>NIFEXQVDAQPLRPCELQRERAFLKREDYVPQCAEDGSFQTVQCGKDGASCWCVDADGREVPGSRQPGRPAACLSFCQLQKQQILLSSYINSTATSYLPQCQDSGDYSPVQCDLRRRQCWCVDAEGMEVYGTRQQGRPARCPRSCEIRNRRLLHGVGDRSPPQCSPDGAFRPVQCKFVNTTDMMIFDLVHSYSRFPDAFVTFSSFRSRFPEVSGYCYCADSQGRELAETGLELLLDEIYDTIFAGLDLASTFAETTLYRILQRRFLAVQLVISGRFRCPTKCEVERFAATSFRHPYVPSCHPDGEYQAAQCQQGGPCWCVDSRGQEIPGTRQRGEPPSCAEDQSCPSERRRAFSRLRFGPSGYFSRRSLLLAPEEGPVSQRFARFTASCPPSIKELFLDSGIFQPMLQGRDTRFVAPESLLKEAIRGLFPSRELARLALQFTTNAKRLQQNLFGGRFLVNVGQFNLSGALGTRGTFNFSHFFQQLGLPGFQDGRALADLAKPLSVGLNSNPASEAPKASKIDVALRKPVVGSFGFEVNLQENQNALQFLSSFLELPEFLLFLQHAISVPEDIARDLGDVMEMVFSSQGCGQAPGSLFVPACTAEGSYEEVQCFAGDCWCVDAQGRELAGSRVRGGRPRCPTECEKQRARMQSLLGSQPAGSSLFVPACTSKGNFLPVQCFNSECYCVDTEGQPIPGTRSALGEPKKCPSPCQLQAERAFLGTVRTLVSNPSTLPALSSIYIPQCSASGQWSPVQCDGPPEQAFEWYERWEAQNSAGQALTPAELLMKIMSYREAASRNFRLFIQNLYEAGQQGIFPGLARYSSFQDVPVSVLEGNQTQPGGNVFLEPYLFWQILNGQLDRYPGPYSDFSAPLAHFDLRSCWCVDEAGQKLEGTRNEPNKVPACPGSCEEVKLRVLQFIREAEEIVTYSNSSRFPLGESFLAAKGIRLTDEELAFPPLSPSRETFLEKFLSGSDYAIRLAAQSTFDFYQRRLVTLAESPRAPSPVWSSAYLPQCDAFGGWEPVQCHAATGHCWCVDGKGEYVPTSLTARSRQIPQCPTSCERLRASGLLSSWKQAGVQAEPSPKDLFIPTCLETGEFARLQASEAGTWCVDPASGEGVPPGTNSSAQCPSLCEVLQSGVPSRRTSPGYSPACRAEDGGFSPVQCDPAQGSCWCVLGSGEEVPGTRVAGSQPACESPQCPLPFSVADVAGGAILCERASGLGAAAGQRCQLRCSQGYRSAFPPEPLLCSVQRRRWESRPPQPRACQRPQFWQTLQTQAQFQLLLPLGKVCSADYSGLLLAFQVFLLDELTARGFCQIQVKTAGTPVSIPVCDDSSVKVECLSRERLGVNITWKLQLVDAPPASLPDLQDVEEALAGKYLAGRFADLIQSGTFQLHLDSKTFSADTSIRFLQGDRFGISPRTQFGCLEGFGRVVAASDASQDALGCVKCPEGSYFQDEQCIPCPAGFYQEQAGSLACVPCPEGRTTVYAGAFSQTHCVTDCQKNEVGLQCDQDGQYRASQRDRTSGKAFCVDGEGRRLPWTEAEAPLVDAQ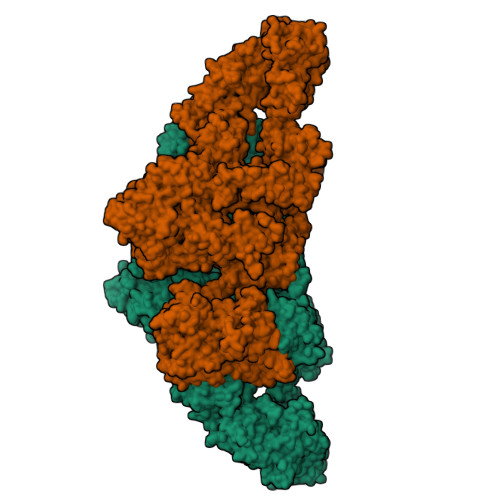CLVMRKFEKLPESKVIFSADVAVMVRSEVPGSESSLMQCLADCALDEACGFLTVSTAGSEVSCDFYAWASDSIACTTSGRSEDALGTSQATSFGSLQCQVKVRSREGDPLAVYLKKGQEFTITGQKRFEQTGFQSALSGMYSPVTFSASGASLAEVHLFCLLACDHDSCCDGFILVQVQGGPLLCGLLSSPDVLLCHVRDWRDPAEAQANASCPGVTYDQDSRQVTLRLGGQEIRGLTPLEGTQDTLTSFQQVYLWKDSDMGSRSESMGCRRDTEPRPASPSETDLTTGLFSPVDLIQVIVDGNVSLPSQQHWLFKHLFSLQQANLWCLSRCAGEPSFCQLAEVTDSEPLYFTCTLYPEAQVCDDILESSPKGCRLILPRRPSALYRKKVVLQDRVKNFYNRLPFQKLTGISIRNKVPMSDKSISSGFFECERLCDMDPCCTGFGFLNVSQLKGGEVTCLTLNSLGLQTCSEEYGGVWRILDCGSPDTEVRTYPFGWYQKPVSPSDAPSFCPSVALPALTENVALDSWQSLALSSVIVDPSIRNFDVAHISTAAVGNFSAARDRCLWECSRHQDCLVTTLQTQPGAVRCMFYADTQSCTHSLQAQNCRLLLHEEATYIYRKPNIPLPGFGTSSPSVPIATHGQLLGRSQAIQVGTSWKPVDQFLGVPYAAPPLGEKRFRAPEHLNWTGSWEATKPRARCWQPGIRTPTPPGVSEDCLYLNVFVPQNMPPNASVLVFFHNAAEGKGSGDRPAVDGSFLAAVGNLIVVTASYRTGIFGFLSSGSSELSGNWGLLDQVVALTWVQTHIQAFGGDPRRVTLAADRGGADIASIHLVTTRAANSRLFRRAVLMGGSALSPAAVIRPERARQQAAALAKEVGCPSSSVQEMVSCLRQEPARILNDAQTKLLAVSGPFHYWGPVVDGQYLRETPARVLQRAPRVKVDLLIGSSQDDGLINRAKAVKQFEESQGRTSSKTAFYQALQNSLGGEAADAGVQAAATWYYSLEHDSDDXASFSRALEQATRDYFIICPVIDMASHWARTVRGNVFMYHAPESYSHSSLELLTDVLYAFGLPFYPAYEGQFTLEEKSLSLKIMQYFSNFIRSGNPNYPHEFSRRAPEFAAPWPDFVPRDGAESYKELSVLLPNRQGLKKADCSFWSKYIQSLKASADETKDGPSADSEEEDQPAGSGLTEDLLGLPELASKTYSK[2x]>SPSSGLGSITDLLNNILSVANQIIYNSAVALPLQLDTLESTLLTAIKSLQTSDKLEQNCSWSAALINDNRYINGINQFYFSIAEGRNLTLGPLLNMPSFIPTATTPEGCTRIPSFSLTKTHWCYTHNVILNGCQDHVSSNQFVSMGIIEPTSAGFPFFRTLKTLYLSDGVNRKSCSISTVPGGCMMYCFVSTQPERDDYFSAAPPEQRIIIMYYNDTIVERIINPPGVLDVWATLNPGTGSGVYYLGWVLFPIYGGVIKGTSLWNNQANKYFIPQMVAALCSQN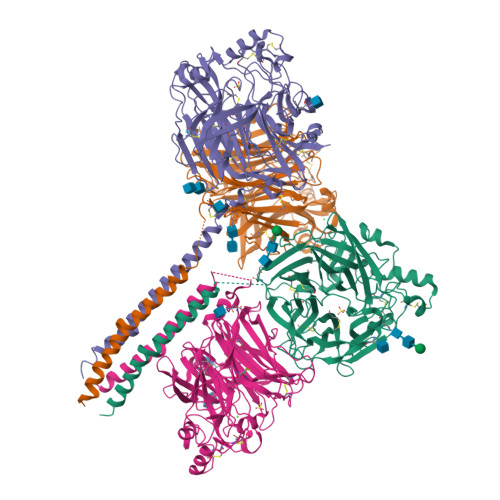QATQVQNAKSSYYSSWFGNRMIQSGILACPLRQDLTNECLVLPFSNDQVLMGAEGRLYMYGDSVYYYQRSNSWWPMTMLYKVTITFTNGQPSAISAQNVPTQQVPRPGTGDCSATNRCPGFCLTGVYADAWLLTNPSSTSTFGSEATFTGSYLNTATQRINPTMYIANNTQIISSQQFGSSGQEAAYGHTTCFRDTGSVMVYCIYIIELSSSLLGQFQIVPFIRQVTLS[4x]> MVTKVLLVSLALFALGTCQVAVNLCTQYGWPNGNYPDPYDCRKYISCNGAVATVMSCALGTVFNPNTRNCDAYGNVPICQYALPSPIVVTNICNQYGWGNGNFYHPYNCAEYIGCANGLTTVNACGAGQYYDQALGRCALAGTGYCRQYVFTPPPAPVVYPDGFDTYC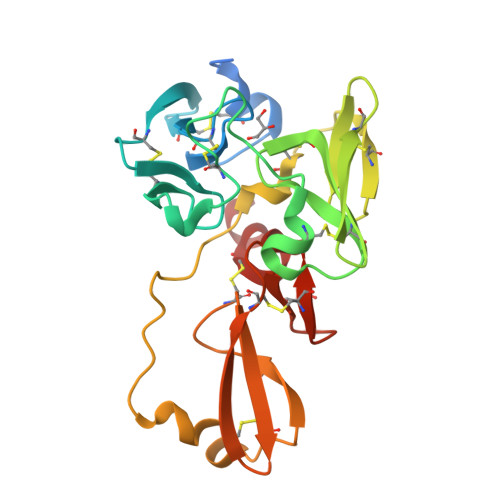SANNLATGIHPDPYSCFSYVECTFGRTTHMPCPAGLSFDRSLLVCDGNRYQNCGGNVLVGK> RSCI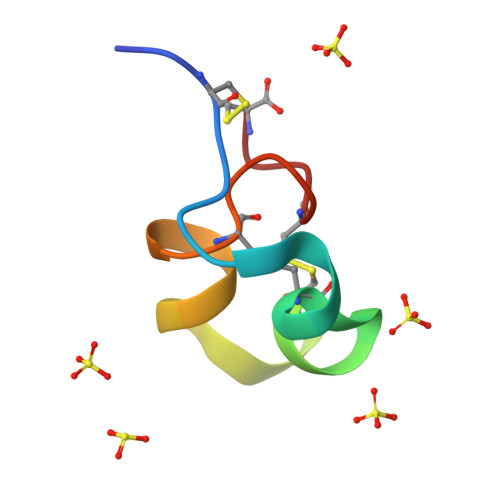DTIPKSRCTAFKCKHSMKYRLSFCRKTCGTC>[5x]MGSSHHHHHHSSGLVPRGSTQAHRSAALVNQANTAMLEDSARQRLQAHAETQALRIQRYFMDAYQYGNGFARLVQVLKDRGGSDLRAELTRQARASLAGNPDVIGLYLVFQPNALDQQDSHYLGQDAMGSNESGRFSLYWSQPSPGTLELEAMPETMLGDTSIGSNGAAKNRWLTCPQDTARTCMLEPYLDEVNGRQVLMTSIALPLL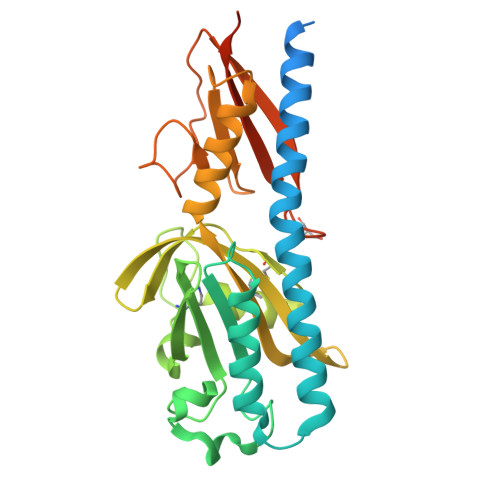EHGKVVGVVGLDIGLANLQQLSVNGRRDLFDGQGQVSIATAAGLLAGNSRDDSVLGKPMDKSVADGLLRVAHPFTPIPDTAPWQVVLELPESVLQAPAVALNQRLDAHNQNAN>KEGQTEVKTVYAQNVIAPNTLSNSIRMLGSQSPLIQAYGLVILQQPDIKVNAMSSLTNHQKFAKANVREWIDEYNPKLIDLNQEMMRYSIRFNSYYSKLYELAGNINEDEQSKADFTNAYGKLQLQVQSIQENMEQDLLELNRFKTVLDKDSNNLSIKADEAIKTLQGSSGDIVKLREDIKRIQGEIQAELTTILNRPQEIIKGSINIGKQVFTITNQTAQTKTIDFVSIGTLSNEIVNAADSQTREAALRIQQKQKELLPLIQKLSQTEAEATQITFVEDQVSSFTELIDRQITTLETLLTDWKVL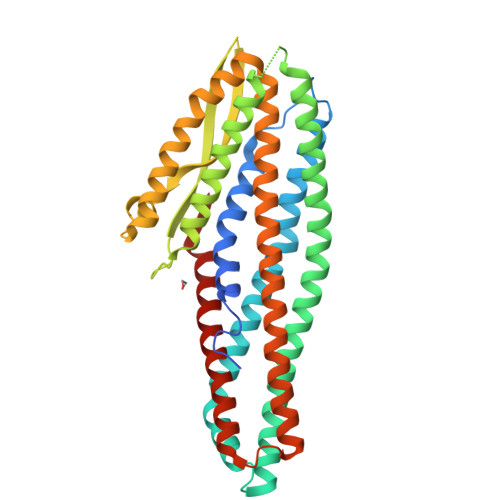NNNMIQIQKNVEEGTYTDSSLLQKHFNQIKKVSDEMNKQTNQFEDYVTNVEVH[8x]> SPWYYGKVTRHQAEMALNERGHEGDFLIRDSESSPNDFSVSLKAQGKNKHFKVQLKETVY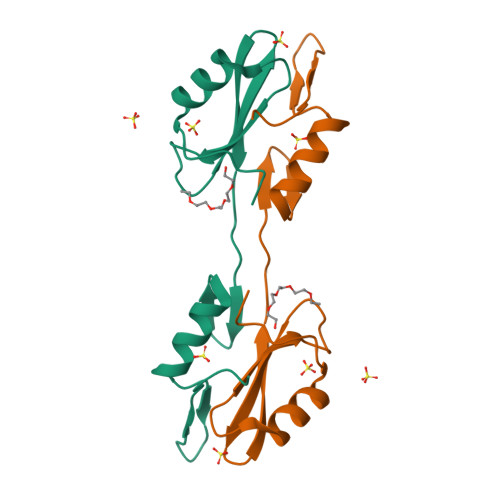CIGQRKFSTMEELVEHYKKAPIFTSEQGEKLYLVKHLSS>GPHMSFNKNGCLVFVSRLWDLDKLGMFHHPVSAEELPDYHTVIKRPVDLSSIRDGIEKGTYATDVDVQNDVARMITNALEYNAKGSTWYQEAMS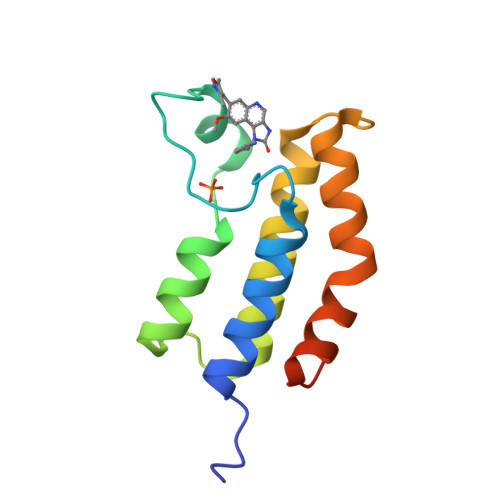FRKTYLDLARQSGLVVDDDEAYIPS[2x]>EEGQKVDHCARHGEKLLLFCQEDSKVICWLCERSQEHRGHHTFLMEEVAQEYHVKLQTALEMLRQKQQEAETERNQVAKRVPKAPPEEKEALIARGKALGEQTQYMRELISELEHRLQGSMMDLLQGVDGIIKRIENMTLK[2x]

TRIM5α is a restriction factor that intercepts the incoming capsids of diverse retroviruses, including HIV-1, and inhibits viral replication. Like all TRIM proteins, TRIM5α consists of an N-terminal tripartite or RBCC motif (RING, B-box 2, and coiled-coil domains), followed by a C-terminal domain. Higher-order assembly of TRIM5α requires the B-box 2 domain, which is thought to mediate three-fold symmetric interactions that connect coiled-coil mediated TRIM5α dimers into a hexagonal net. We therefore engineered artificial constructs – which we call miniTRIMs – that retain the integrated B-box/coiled-coil fold of the full-length dimer but are more amenable to biochemical and structural analyses.

A P212121 crystal contained two trimers in the asymmetric unit (3.26 Å resolution, R/Rfree = 0.26/0.30), a C2 form contained one dimer (2.1 Å, R/Rfree = 0.18/0.22), and a P1 form contained two dimers (2.3 Å, R/Rfree = 0.22/0.26). Interestingly, the majority of Bcc miniTRIM crystals we obtained (including three other forms that we did not refine) were composed of dimers. The dimer is quasi-equivalent to the trimer: the same sets of residues make the same interactions but with valence of two instead of three. The dimer buries a smaller surface area per subunit (450 Å2) compared to the trimer. Comparison of the trimer and dimer bonding interactions revealed that the two oligomers are distinguished primarily by intermolecular packing between the Trp117, Leu118, and Leu132 sidechains in the hydrophobic layer. In particular, Leu118 and Leu132, which are located at the outer edges of the binding surface, are in van der Waals contact in the trimer, but more separated in the dimer. Another distinction is that the first two turns of the coiled-coil helix are overwound and bent in the dimer form, which might indicate some structural communication between the interacting B-boxes and the coiled-coil domain. Thus, the Bcc miniTRIM was predominantly dimeric in solution. In context of the full-length protein, assembly cooperativity drives the B-box into the trimer form, and so the B-box dimer might represent an intermediate state that can incorporate an additional B-box domain to form the trimer.> MHHHHHHSSGRENLYFQGADLVPPPGYYAAVGERKGSAGSCPAVPPPYTGSLVFTSAYEGSDSARATLNVKAEKTFRSQIKDITDMERGATKLVTQYMRSGRDGDLACALNWMSAWARAGALQSDDFNHTGKSMRKWALGSLSGAYMRLKFSSSRPLAAHAEQSREIEDWFARLGTQVVRDWSGLPLKKINNHSYWA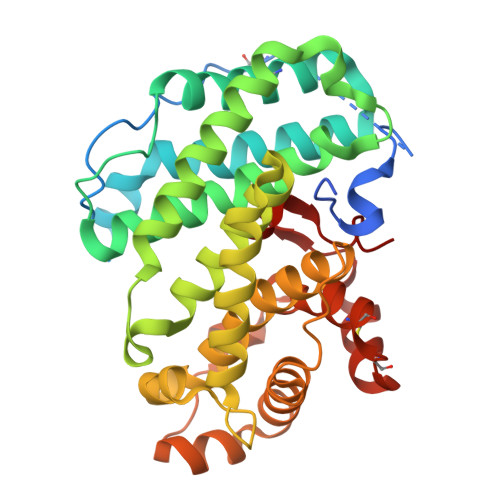AWSVMSTAVVTNRRDLFDWAVSEFKVAANQVDEQGFLPNELKRRQRALAYHNYALPPLAMIAAFAQVNGVDLRQENHGALQRLAERVMKGVDDEETFEEKTGEDQDMTDLKVDNKYAWLEPYCALYRCEPKMLEAKKDREPFNSFRLGGEVTRVFS5-[3-(3-fluorophenoxy)propoxy]quinazoline-2,4-diamine 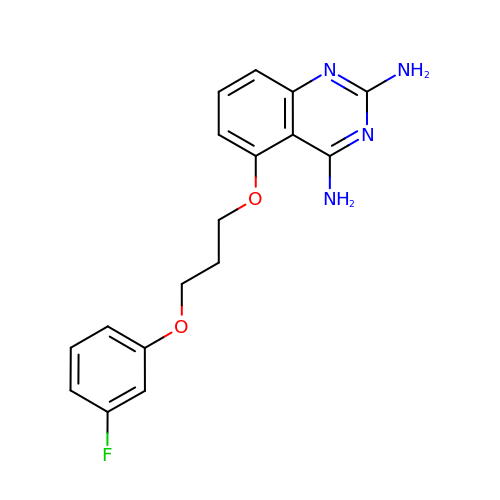| C17 H17 F N4 O2 | WYNJMQXBACXTGZ-UHFFFAOYSA-N> MLNLLKSWLKNSLMAILLVTIFLGINTAGWTPSSNAALPSGNAITDGRALLRYALPINNKPVRELQASLEDISAQLRANRRWGAVSKDLSKASRILDKPSQILTSVPEERQTQAETWINELKTGVVKVQELAQSKDKEQVLLE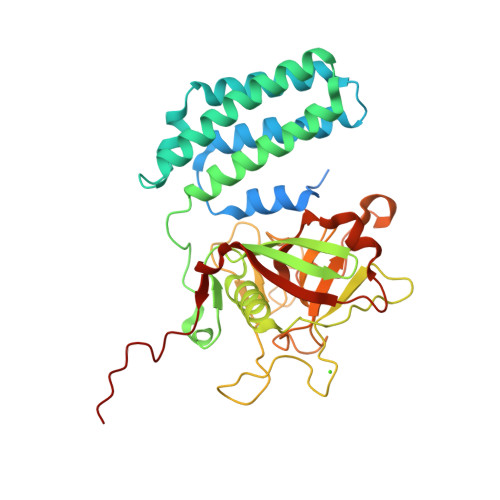RAKLLNLVSLIEESMVKEFPFEVPEEYNNLPQLKGRATIAIKTNKGDLTVVVDGYSAPVTAGNFVDLVKRGFYNGLEFTRSEESYVLQTGDPPGKEQGFIDPKTGKYRAIPLEILAEGDKKPTYGITLEDAGRYLDMPVLPFSSFGALAMARPETEVDGASSQVFFFLFEPELTPAGRNLLDGRYSVFGYLIEGRDILDTLKAGDKIESATVVQGLDNLVQPQSAAIEVLFQ> GAMVDIPLRLLVP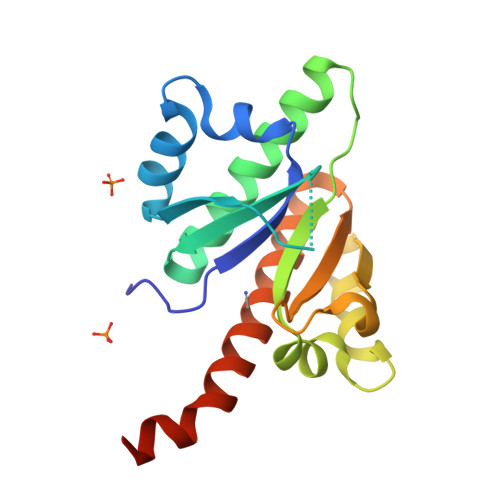TQYVGAIIGKEGATIRNITKQTQSKIDVHRKENAGAAEKAISVHSTPEGCSSACKMILEIMHKEAKDTKTADEVPLKILAHNNFVGRLIGKEGRNLKKVEQDTETKITISSLQDLTLYNPERTITVKGAIENCCRAEQEIMKKVREAYENDVAAMSLQSHLIPGLN3,3-bis(4-hydroxyphenyl)-2-benzofuran-1-one 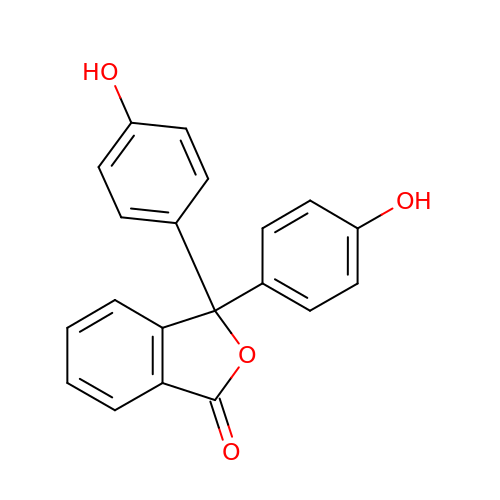| C20 H14 O4 | KJFMBFZCATUALV-UHFFFAOYSA-N>[3x]GHHHHHHEDGETKTEQTA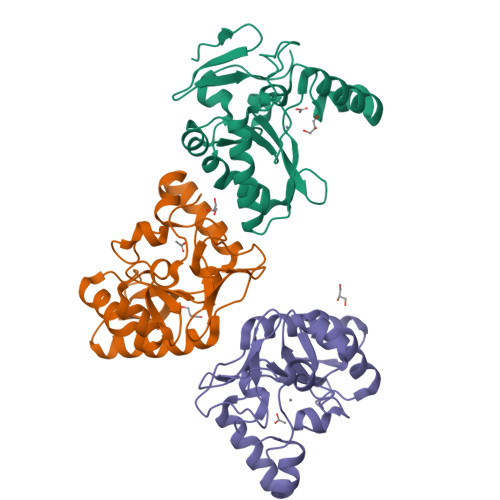KADGTVGSKSQGAAQKKAEVVNKGDYYSIQGKYDEIIVANKHYPLSKDYNPGENPTAKAELVKLIKAMQEAGFPISDHYSGFRSYETQTKLYQDYVNQDGKAAADRYSARPGYSEHQTGLAFDVIGTDGDLVTEEKAAQWLLDHAADYGFVVRYLKGKEKETGYMAEEWHLRYVGKEAKEIAASGLSLEEYYGFEGGDYVD AAC(2′)-Ia is chromosomally restricted in Providencia stuartii, an opportunistic pathogen responsible for catheter-associated urinary tract infections with a high mortality rate. This enzyme is a part of a larger group of AAC(2′)-I isozymes, which includes five enzyme subtypes (AAC(2′)-Ia—AAC(2′)-Ie). Specifically, AAC(2′)-Ia utilizes cosubstrate, acetyl-CoA, to detoxify naturally occurring aminoglycosides such as kanamycin, tobramycin, sisomicin, and gentamicin, as well as semisynthetic aminoglycosides such as dibekacin, netilmicin, and plazomicin through the addition of an acetyl group at their 2′ positions.

Meanwhile, the crystal structures of AAC(2′)-Ia in complex with CoA and acetylated aminoglycosides describes the enzyme in three product-bound states. While the aminoglycoside portion of acetylated-gentamicin only hydrogen bonds with AAC(2′)-Ia via three residues, the tobramycin moiety can interact with up to 7 residues. In identical fashion to gentamicin, the central ring of tobramycin is anchored by two hydrogen bond interactions, N-1 with Glu149 and N-3 with the C-terminal carboxylate of Trp178. Additionally, both aminoglycosides interact with the backbone carbonyl of Ser114 at their site of modification, N-2′. Aside from these interactions, the prime-ring of tobramycin also interacts with the backbone carbonyl of Asp32 and the side chain of Asp37 at the N-6′ position. At the double-prime ring, tobramycin interacts with the enzyme at its N-4′′ and O-5′′ via hydrogen bond with Asp117. The tobramycin molecule in chain B also forms an additional hydrogen bond interaction between its O-2′′ and Glu148 of AAC(2′)-Ia. The acetyl group modification of the molecule interacts with the enzyme by way of the backbone amine of Met81. The acetylated tobramycin in chain A also interacts with the backbone amine of the adjacent residue, Ala80. In the tobramycin-bound structure, there is no chemical addition at the N-1 amine, and therefore Glu148 can adopt either conformation.

>MGIEYRSLHTSQLTLSEKEALYDLLIEGFEGDFSHDDFAHTLGGMHVMAFDQQKLVGHVAIIQRHMALDNTPISVGYVEAMVVEQSYRRQGIGRQLMLQTNKIIASCYQLGLLSASDDGQKLYHSVGWQIWKGKLFELKQGSYIRSIEEEGGVMGWKADGEVDFTASLYCDFRGGDQW[2x]Many parasitic Orobanchaceae have evolved a large clade of diversified KAI2 proteins (KAI2d) as receptors for exogenous strigolactones. We present the genome of Castilleja foliolosa, which reveals an abundance of KAI2d paralogs that act as strigolactone receptors. Castilleja foliolosa’s KAI2d proteins include high-turnover enzymes, in particular KAI2d15, which features a substrate binding pocket with a methionine cluster at its entrance that is involved in the trade-off between substrate turnover and affinity. In summary, our research reveals that Castilleja possesses a large clade of KAI2d proteins, acting as strigolactone receptors, participating in activating a parasitic state in the plant.

To obtain additional insight into the strigolactone perception in Castilleja, we solved the crystal structure of KAI2d15 at a resolution of 1.8 Å. As expected, the protein adopted a canonical α/β hydrolase architecture, with a 4-helix lid domain covering the substrate binding pocket containing a Ser/His/Asp catalytic triad at its base. The substrate binding pocket was quite voluminous, measuring 908 Å3, which surpassed the 861 Å3 found in the strigolactone receptor KAI2d4 from Orobanche minor, but was smaller than the 1111 Å3 detected in the highly sensitive SL receptor HTL7 from Striga hermonthica. We found 3 methionine residues in the crystal structure of KAI2d15 that surround the entrance to the protein’s substrate binding pocket, including an alternative side-chain conformation of M142. To study the effect of these methionine residues on the receptor’s substrate specificity and sensitivity, we created a protein variant, replacing the three methionines with valines (KAI2d15 M142V M153V M157V). The mutant protein showed destabilization at lower ligand concentrations when GR24 or 5-deoxystrigol were present, while the wild-type protein destabilized at lower concentrations of strigol or orobanchol. We specifically compared Michaelis-Menten parameters between the KAI2d15 wild type and the mutant, in which three of the methionines at the substrate pocket entrance had been replaced with valines (KAI2d15 M142V M153V M157V). While the turnover numbers (kcat) of these proteins showed no significant difference, we found a 3-fold decrease in the Michaelis constant (KM) for wild-type KAI2d15 as compared to the mutant version (0.8 μM in wild-type KAI2 vs. 2.4 μM in KAI2d15 M142V M153V M157V). We observed a linear trade-off between these two catalytic parameters in all investigated KAI2 proteins, except KAI2d15, and remarkably, the trade-off was restored in the KAI2d15 M142V M153V M157V mutant. Thus, a possible dual role of the methionines in both enhancing substrate binding and promoting product release might be the molecular basis for KAI2d15 mitigating the typical trade-off observed in enzyme kinetics.

>GPMSTIGATHNVRVVGSGRKTIVLGNGYGTDQSVWRHLVPHLVGRYKVLLYDNMGAGTTNPDYYDFDRYATLEGFAYDLLAILEEFNVRKCIYVGHSMAAMVGMIASIFRPDLFHKLITISATPRMSNTDDYYGGFEQEELDQMDEGLRMNHESMIRGMAPLVVGGDMDSEAVHEYTRMLLNMRPDIALSLSRTLYAFDMRPFLGQVTVPCHILQSSKDMGVPVAVAEYLHQSLGGKSIVEVMSAEGHLPHLSAPEITIPVLLRHIQQDI[2x]>[2x]SMLKLSAENESTPIQQLLEHFLRQLQRKDPHGFFAFPVTDAIAPGYSMIIKHPMDFGTMKDKIVANEYKSVTEFKADFKLMCDNAMTYNRPDTVYYKLAKKILHAGFKMMSKERLLALKRSMS

Bromodomains (BRDs) are protein interaction modules that selectively recognize ε-N-lysine acetylation motifs, a key event in reading the posttranslational modifications that constitute the epigenetic code. The closely related BRDs BRD7 and BRD9 are part of the SWI/SNF nucleosome-remodeling complex, which plays a crucial role regulating gene expression programs, including the expression of inflammatory genes. Although BRDs share similar acetyl–lysine recognition motifs, there are significant differences in distal parts of the binding pocket. Owing to a shift in the ZA loop in BRD9, this region is much larger in BRD9, with residues A46, F47, P48, T50, and I53 forming a large hydrophobic cavity.

The C7 position was viewed as an ideal attachment point for a structurally complex heterocyclic appendage that could exploit this cavity for selective inhibition of BRD9. Furthermore, analysis of the BRD9/1 model suggested that a C4 methyl group on the quinolone would occupy a shallow hydrophobic pocket, thereby increasing potency. Changes in the melting temperatures (ΔTm) confirmed that nearly all of the elaborated quinolones were tolerated, and valerolactam 6 was selected as a lead structure for further characterization and optimization. Co-crystallization with BRD9 showed the conserved H bonding of acetyl–lysine recognition: Compound 6 exhibited H bonds to N100 and to a conserved water molecule. The valerolactam moiety extends into the desired hydrophobic region between F44 and I53 whilst positioning the amide carbonyl near, but not in H bond contact with, Y106. Furthermore, the introduced methyl group at the C4 position demonstrated additional hydrophobic interactions with A54 and Y106. ITC confirmed the activity determined by the DSF assay: 6 bound to BRD9 with a dissociation constant (KD) of 612 nm.>MRNQDKRAAHKDSEPSTEVNHTASSYQGRQQETGMNLRGIDGNEPTEGSNLLNNNEKMQGTPAEPNHLQRRRQIHACPPRGLLARVITNVTMVILLWAVVWSVTGSECLPGGNLFGIIMLFYCAIIGGKLFGLIKLPTLPPLPPLLGMLLAGFLIRNVPVISDNIQIKHKWSSALRSIALSVILVRAGLGLDSNALKKLKGVCVRLSLGPCLIEACTSAVLAYFLMGLPWQWGFMLGFVLGAVSPAVVVPSMLLLQEGGYGVEKGIPTLLMAAGSFDDILAITGFNTCLGMAFSTGSTVFNVLKGVLEVIIGVVTGLVLGFFIQYFPSSDQDNLVWKRAFLVLGLSVLAVFSSTYFGFPGSGGLCTLVTAFLAGRGWASTKTDVEKVIAVAWDIFQPLLFGLIGAEVLITALRPETIGLCVATLGIAVLIRILVTYLMVCFAGFNIKEKIFISFAWLPKATVQAAIGSVALDTARSHGEKQLEGYGMDVLTVAFLSIIITAPVGSLLIGLLGPRLLQKAEQNKDEEDQGETSIQV[2x]

The Na+/H+ exchanger SLC9B2, also known as NHA2, correlates with the long-sought-after Na+/Li+ exchanger linked to the pathogenesis of diabetes mellitus and essential hypertension in humans. Here we report the cryo-EM structures of bison NHA2 in detergent and in nanodiscs, at 3.0 and 3.5 Å resolution, respectively. NHA2 consists of 14 transmembrane (TM) segments, rather than the 13 TMs previously observed in mammalian Na+/H+ exchangers (NHEs) and related bacterial antiporters. The additional N-terminal helix in NHA2 forms a unique homodimer interface with a large intracellular gap between the protomers, which closes in the presence of phosphoinositol lipids.

The bison NHA2 construct used for structural studies is referred to as NHA2ΔN, because it does not include the first 69 residues of the N-terminal tail. The bison NHA2ΔN sample preparation was subsequently optimized for grid preparation, cryo-EM data acquisition and structural determination at pH 8.0. The final cryo-EM map of NHA2ΔN in detergent was estimated at 3.0 Å (Fourier shell correlation (FSC) = 0.143 criterion), although protomer A was consistently better aligned than protomer B, and was therefore resolved at a higher resolution. The observed additional N-terminal helix TM –1 is part of the dimer domain in NHA2ΔN and is domain-swapped, mediating homodimerization by interacting with TM8 and the TM8–TM9 loop in the neighboring protomer. As a result of the tilted angle of TM –1 and the length of the connecting loop to TM1, the NHA2ΔN protomers are held apart by ~ 25 Å on the intracellular side. Before masked refinement we also observed additional map density for a predicted short helical segment prior to TM −1, which sits at right angles to the protein. Finally, the modeled N-terminal extension helix is also highly positively charged and is reminiscent of the positively charged extension helix seen in the oligomeric betamine transporter BetP, which binds to negatively charged lipids in response to a change in cell volume.Toxoplasma gondii is one of the most significant parasites that impacts human health, with estimates that as many as one third to one half of the human population are infected. At the Center for Structural Genomics of Infectious Diseases (CSGID), the first Toxoplasma Structural Genomics Pipeline was established. The enzymes selected from the TDR database as small and tractable for expression and crystallization included: phosphoglycerate mutase II (hereafter referred to as PGM), nucleotide diphosphate kinase (NDK), ribulose phosphate 3-epimerase (RPE), ribose-5-phosphate isomerase (RPI), and ornithine aminotransferase (OAT). The genes encoding these enzymes were cloned, proteins expressed and purified, crystallized, and crystal structures were determined.

Nucleotide diphosphate kinase catalyzes the movement of phosphate from a nucleoside triphosphate to a nucleoside diphosphate (e.g., GTP + ADP –> GDP + ATP). In both structures, TgNDK forms a hexamer with an average BSA of ~18,900 Å2. Comparison of TgNDK with known crystal structures of homologs proteins suggests that the TgNDK hexamer is likely a biologically functional assembly. TgNDK adopts an α/β/α sandwich fold with four β strands and eight surrounding α helices. The side chain of Tyr160 is spatially positioned in a nucleotide base-binding pocket of the active site of a symmetry-related molecule (not shown). Crystal structure of TgNDK suggests that the protein forms a hexamer with conserved nucleotide binding sites. Pairwise structural alignment revealed that active site of TgNDK may undergo similar conformational changes as its closest homolog, humanNM23-H2 transcription factor. On the other hand, when the dinucleotide is absent, the active site loop comprising of residues G59-F62 (Tg numbering) is shifted significantly (3–4 Å) between species. Additionally, TgNDK residue K60 is residue R58 in the human ortholog, offering different hydrogen-bond capacities to putative ligands. These observations suggest opportunities for the selective design of TgNDK inhibitors using structure-based molecular modeling techniques.

>[12x]MAAKQQERTYIMVKPDGVQRGLVSEVIRRFEQRGYKLVALKMKSPDATLLEEHYADLKGKPFFPGLISYMTSGPVVCMVWEGTDVVKQGRRMLGETRPLESNPGTLRGDFCIDVGRNIVHGSDSVESANKEISLWFTPEEICEWTSAQHKWVYEQGENLY>[3x]MDNAWQNTSGWWN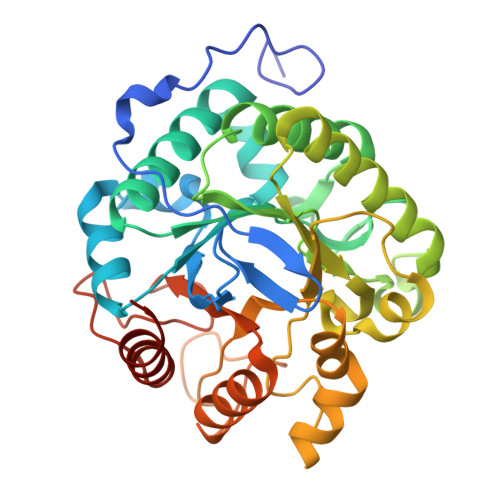AGDVPAFDKRQLSRQLPLIRVDGNRFVDEQGNVQIFRGVSISDPNKLAKDQHFNKKHFDVIRSWGTNVVRIPVHPSAWRERGVKGYLELLDQAITWNNELGMYTIIDWHSMGNLKSEMFQNSMYHTSKGETFDFWRRVSERYNGINSVAFYEIFNEPTVFSGRLGIVSWAEWKAINEEAITIIQAHNPNAISLVAGFNWAYDLREAAANPIERNNVAYVSHPYPQKVGAPYQANWERDFGFMADKYPVFATEIGYQLASDKGAHIPVIDDGSYGPRITDYFAKKGISWVAWVFDPDWSPQMIKSWDYEPTMQGEHFRKVMLKENKLEHHHHHH> DELYRQSLEIISRYLREQATGAKDTKPMGRSGATSRKALETLRRVGDGVQRNHETAFQGMLRKLDIKNEDDVKSLSRVMIHVFSDGVTNWGRIVTLISFGAFVAKHLKTINQESCIEPLAESITDVLVRTKRDWLVKQRGWDGFVEFFH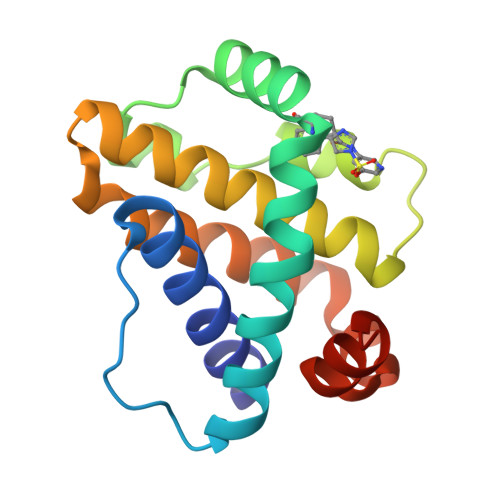VED> MTFAHEVVKSNVKNVKDRKGKEKQVLFN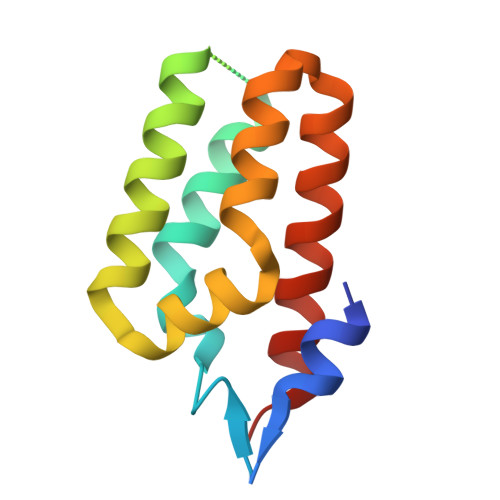GLTTSKLRNLMEQVNRLYTIAFNSNEDQLNEEFIDELEYLKIKFYYEAGREKSVDEFLKKTLMFPIIDRVIKKESKKFFLDYCKYFEALVAYAKYYQKED> GPLGSMEGEELIYHNIINEILVGYIKYYIN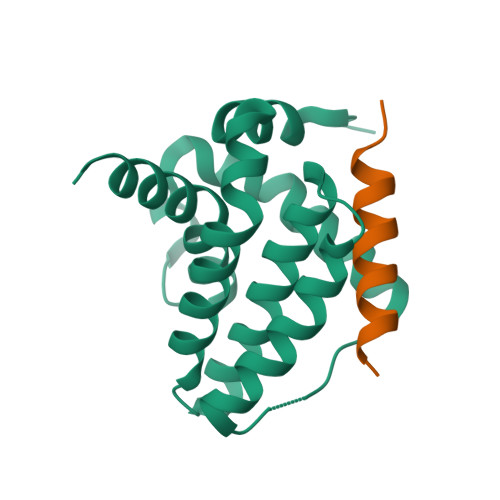DISEHELSPYQQQIKKILTYYDECLNKQVTITFSLTSVQEIKTQFTGVVTELFKDLINWGRICGFIVFSAKMAKYCKDANNHLESTVITTAYNFMKHNLLPWMISHGGQEEFLAFSLHSDMYS;> VPQDASTKKLSECLKRIGDELDSNMELQ6-ETHYL-5-[1-(3-METHOXYPROPYL)-1,2,3,4-TETRAHYDROQUINOLIN-7-YL]-N~4~-(2-PHENYLETHYL)PYRIMIDINE-2,4-DIAMINE | C27 H35 N5 O | 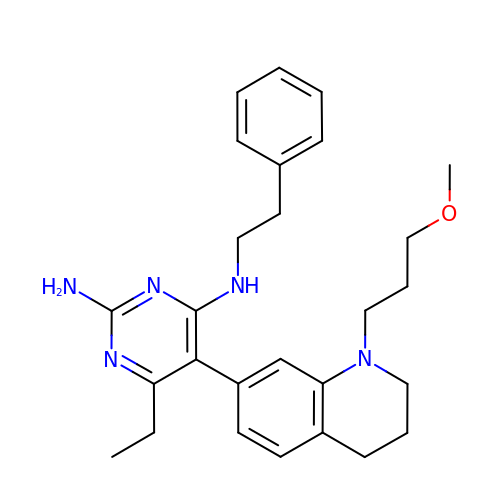DGNIHJBLLNEWQZ-UHFFFAOYSA-N> MDSNTVSSFQVDCFLWHVRKRFADQELGDAPFLDRLRADQASLRGRGNTLGLDIETATRAGKQIVERILEEESDKALKMPASRYLTDMTLEEMSRDWFMLMPKQKVAGSLCIKMDQAIMDKTIILKANFSVIFDRLETLILL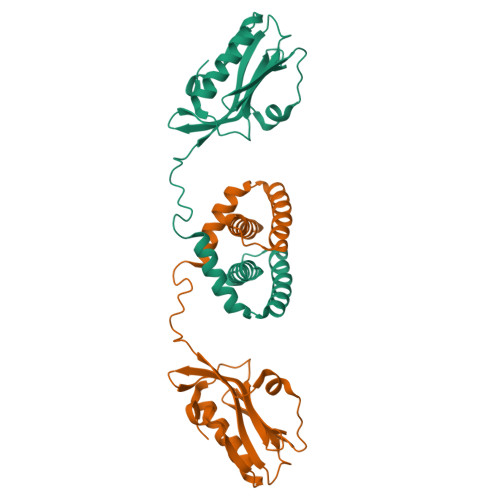RAFTEEGAIVGEISPLPSLPGHTGEDVKNAIGVLIGGLEWNDNTVRVTETIQRFAWRNSDEDGRLPLPPNQKR> AGGGGCGGGGCT;> TAG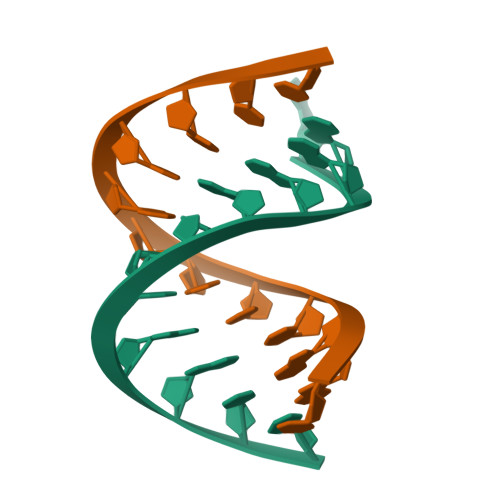CCCCGCCCC>HHHHHHSSGLVPRGSHMLRLGDIAPDFEQDSSEGRIRLHEWLGDSWGVLFSHPADFTPVCTTELGFTAKLKDQFAQRGVKVLALSVDPVDSHLKWIDDINETQDTRVNFPIIADADRKVSELYDLIHPNANDTLTVRSLFIIDPNKKVRLIITYPASTGRNFNEILRVIDSLQLTDEHKVATPANWEDGDEVVIVPSLKDEEEIKRR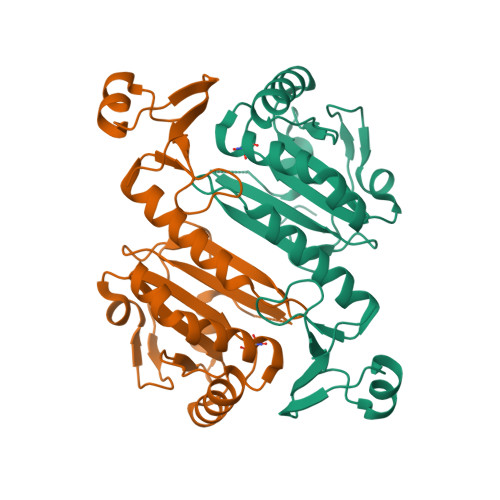FPKGYRAVKPYLRLTPQPNR[2x]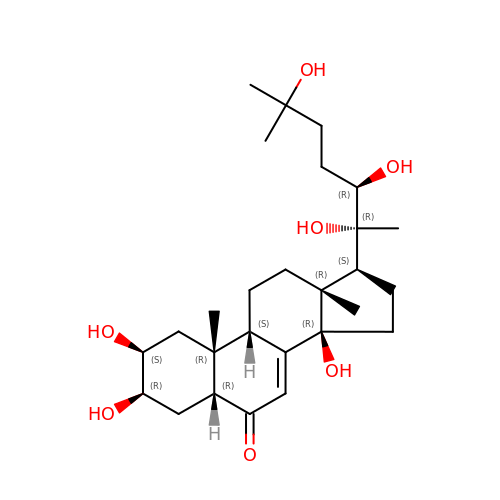(2beta,3beta,5beta,22R)-2,3,14,20,22,25-hexahydroxycholest-7-en-6-one | C27 H44 O7 | NKDFYOWSKOHCCO-YPVLXUMRSA-N N-[4-[[GLUTAMIC ACID]-CARBONYL]-BENZENE-SULFONYL-D-PROLINYL]-3-AMINO-PROPANOIC ACID | C20 H25 N3 O10 S | 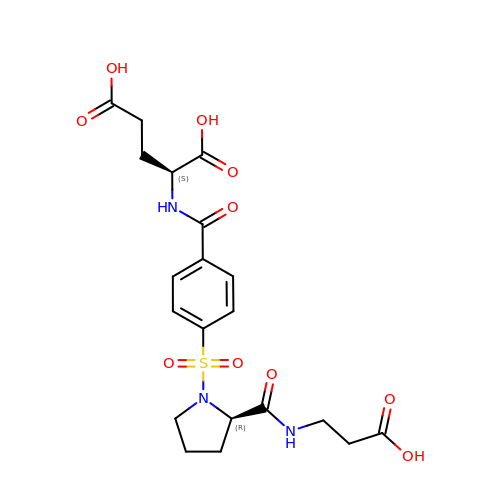SRAHBOKVSSZEHQ-LSDHHAIUSA-N>[15x]MAILGLGTDIVEIARIE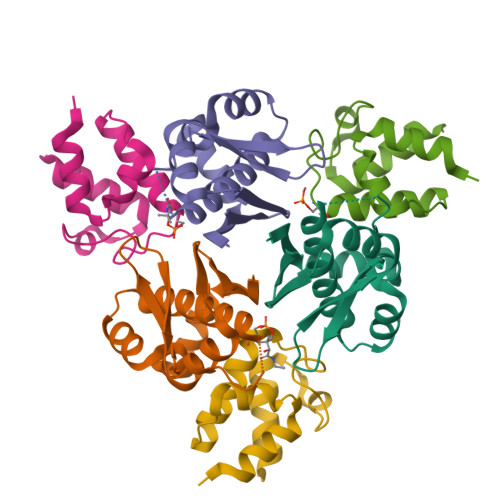AVIARSGDRLARRVLSDNEWAIWKTHHQPVRFLAKRFAVKEAAAKAFGTGIRNGLAFNQFEVFNDELGKPRLRLWGEALKLAEKLGVANMHVTLADERHYACATVIIES;>[15x]MGSTIEERVKKIIGEQLGVKQEEVTNNASFVEDLGADSLDTVELVMALEEEFDTEIPDEEAEKITTVQAAIDYINGHQA(1S)-1-(2-methyl-1,2,4-triazol-3-yl)ethanamine 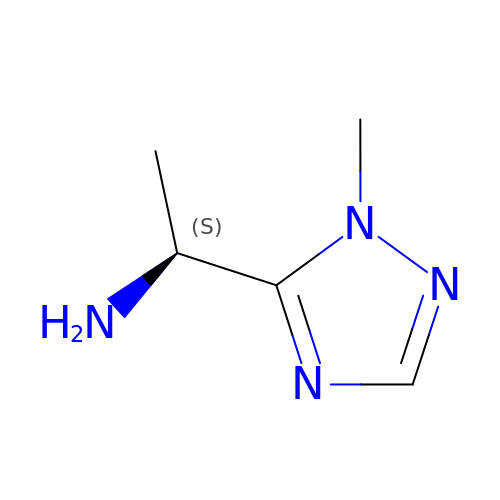| C5 H10 N4 | OCXIKYJPCILJLE-BYPYZUCNSA-N> AVVLPDWYEEAFVNVENLFIDMFTDLLPDYESGCWAPDDWLADEIEVKPTIWFFRL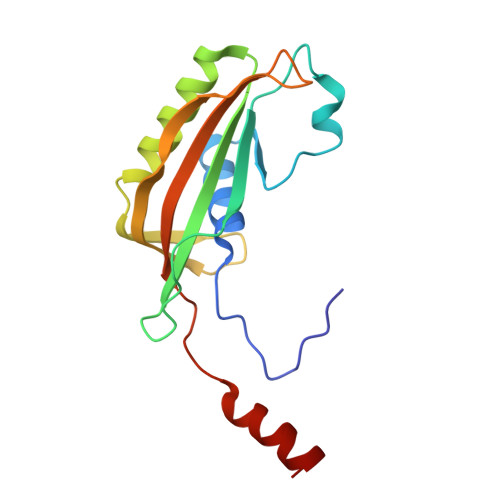PGGRVDWDGRKDECQLQVMVVTGSRDDSWRLMDFVRAMLLPMQGDKYKMADGYTAQIRCAGEVAGPQLLTPGQRIDTRVVTATFKVSVSMKSAKNYKQKLYELWQALRG>[4x]MFITGAFFDILEVGPKKIRRCFELVRVRFAPSPTGHLHVGGARTALFNWMFARKEGGKFILRIEDTDTERSSREYEQQILESLRWCGLDWDEGPDIGGDFGPYRQSERLEIYREYAEKLVEDKRAYYVVYDKEDPSKELFTTYEYPHEYKEKGHPVTIKFKVLPGKTSFEDLLKGYMEFDNSTLEDFIIMKSNGFPTYNFAVVVDDHLMRISHVFRG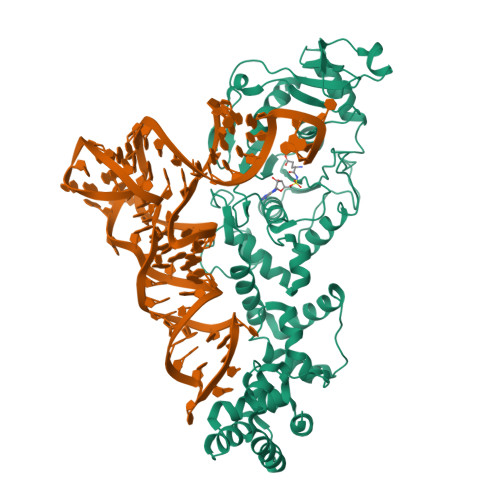EDHLSNTPKQLMIYEAFGWEAPVFMHIPLILGSDRTPLSKRHGATSVEHFRREGILSRALMNYLALLGWRVEGDEIFTIEEKLQSFDPKDISNKGVIFDYQKLEWVNGKHMRRIDLEDLKREFIEWAKYAGKEIPSVDERYFSETLRICREKVNTLSQLYDIMYPFMNDDYEYEKDYVEKFLKREEAERVLEEAKKAFKDLNSWNMEEIEKTLRDLSEKGLASKKVVFQLIRGAVTGKLVTPGLFETIEVLGKERTLKRLERTLQFLKKT> AGFMVPTTNTAGWGRAMAGGSLFPNDPSAAFNNPAAMAFIDKRIAQLTVNYADIDIKYNGDAYDYQGNPMT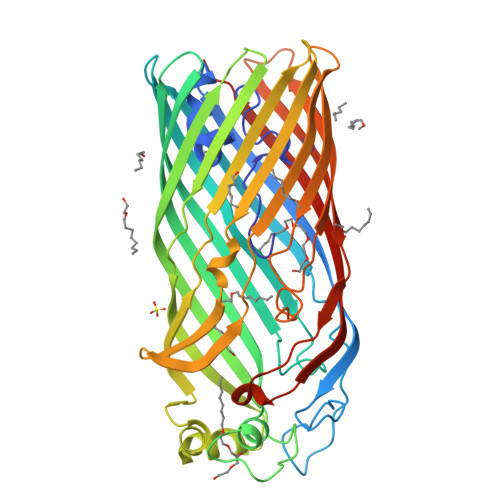GGYQDGPGTPELGTNDGGQAGFGAWLPTGFLVVPINDRFAFGLSQVVPMGMRSTWDPNWKGRDFAVDTKIETIGLTGSLSFKVNDNFSLGAGVIIQRTSGFVSQNLDLYASAANSPGMGGIPFPASNSSALMRVKVDNTSPGFFAGAVWKPTDRDTLGFAYHAKIRNKLKGHYNLYDHDGGLTEGAIEGGTPGLAYPGLDLRMGASASARLDIPAYASLDWVHQFNDRLSLGASATWTEWSSFQDLTLKSHGNTIVSIPYTYRNTWTLAVGGDYKVTDQWTMRAGVAYDQTPTHNATRDPRIPDGDRYFASLGAGYRFQSMPELSIDAAYSRQFVKEVPLKTVNQDRLGGGRLDGRATSKGQVFSLSATYDFHHHHHHHH> TDAFNLVGVGPVSQGMGGIGAAFNIGAQGMMLNPATLTQMQEGMHLGLGMDIITAELEVKNTATGEKADSHSRGRNNGPYVAPELSLVWRGERYALGVGAFASDGVGTQFGDTSFLSRTTTNNLNTGLENYSRLIVLRIPFSAAYQVNEKLSVGASLDAVWTSVNLGLLLDTTQIGTLVGQGQVSGSLMPALLSVPELSAGYLSADNHRASGGGVDSWGIGGRLGLTYQLTPKTRVGIVYNFKTHVGDLSGNADLTAVSAVAGNIPLSGELKLHNFEMPASLVAGISHEFSDQFAVAFDYKRVYWSDVMDDIEVNFKQKATGDTINLKLPFNYRDTNVYSLGAQYRYGANWVFRAGVHYAQLANPSSGTMPIIPSTPTTSLSGGFSYAFSPEDVVDFSLAYGFKKKVSNDSLPITDKPIEVSHSQIVTSISYTKSFHHHHHH

Thus far, only the FadL OM channel family has been shown to mediate transport of hydrophobics. PpF1 has three FadL orthologs, of which TodX (Pput_2883) and CymD (Pput_2901) are located in the adjacent tod and cym/cmt operons respectively. Here we show, by using an integrated approach combining growth assays, X-ray crystallography and molecular dynamics (MD) simulations, that MAH uptake as the first step in biodegradation does occur via lateral diffusion. In the presence of TodX/CymD, robust growth is observed, providing the first direct evidence for MAH transport by FadL-type channels.

To enable similar experiments on CymD, we first determined its crystal structure. Despite considerable efforts, we could only obtain one crystal form that diffracted to sufficient resolution for structure determination. The CymD structure is very similar to that of TodX but lacks density for ~30% of the protein due to mobility of several extracellular loops within the crystal. Importantly however, the visible parts of the structure show that the S2 bulge and the S3 kink are present and in the same location as in TodX. To allow molecular dynamics simulations, we modelled the missing parts of CymD by using the TodX structure as a template. The lateral openings (delineated by the green surface) are similar in size in the wild-type structures of TodX and CymD and differ only slightly from EcFadL, in that the latter does not have a bulge in S2 like TodX and CymD, but a more pronounced kink in S3. Compared to PpF1-3-cymD, PpF1-3-todX grows slightly slower on toluene and clearly does not grow on p-cymene. This suggests that even closely related MAH channels have different specificities, with CymD being able to transport more bulky substrates, such as p-cymene. Growth on p-cymene vapour is observed only with CymD, and the CymD lateral opening mutants have the same phenotypes with toluene and p-cymene. Interestingly, the equivalent sphincter residues in CymD are Ala3, Val106 and Ile373, suggesting that the passage from the P-pocket to the lateral opening is narrower in TodX compared to CymD. Due to the difficulties in crystallising wild-type CymD and its similarity to TodX, no attempts were made to crystallise CymD lateral opening mutants.>SNAMALKKPGSLTIAGSGIASIGHITLETLALIKEADKIFYAVTDPATECYIQENSRGDHFDLTTFYDTNKKRYESYVQMSEVMLRDVRAGRNVLGIFYGHPGVFVAPSHRAIAIAREEGFQAKMLPGISAEDYMFADLGFDPSTYGCMTQEATELLVRNKKLDPSIHNIIWQVGSVGVDTMVFDNGKFHLLVERLEKDFGLDHKIQHYIGAILPQSVTVKDTFAIRDLRKEEVLKQFTTTSTFYVPPRTPAPIDPKAVQALGLPATVTKGAQDWTGFQSVSPAYGPDEMRAVAALDSFVPSQEKAVVHASRAMQSLMVDLALRPALLE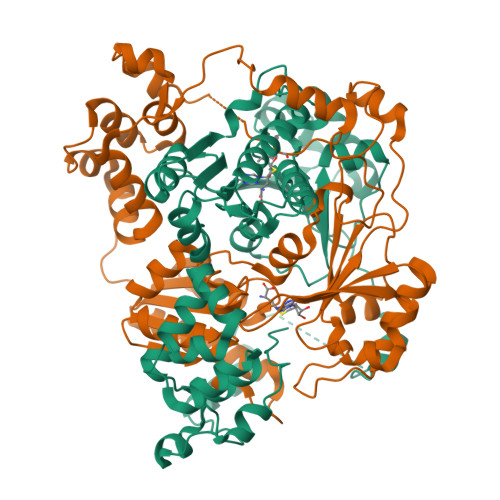QYKADPVAFANTRNGLTAQEKFALGLKKPGPIFVVMRQLPSAIASGQEPSQEEIARADDATALVLAALLVIVG[4x]>MSLINTKIKPFKNQAFKNGEFIEITEKDTEGRWSVFFFYPADFTFVCPTELGDVADHYEELQKLGVDVYAVSTDTHFTHKAWHSSSETIAKIKYAMIGDPTGALTRNFDNMRE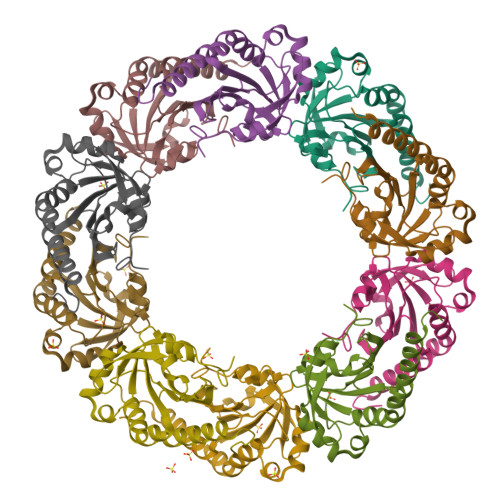DEGLADRATFVVDPQGIIQAIEVTAEGIGRDASDLLRKIKAAQYVASHPGEVCPAKWKEGEATLAPSLDLVGKYFSKHN[10x]> ADTIVAVELDSYPNTDIGDPNYPHIGIDIKSIRSKSTARWNMQTGKVGTVHISYNSVAKRLSAVVSYSGSSSTTVSYDVDL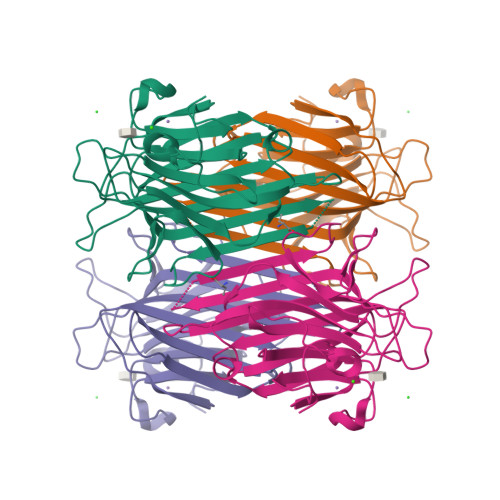NNVLPEWVRVGLSATTGLYKETNTILSWSFTSKLKTNSIADENSLHFSFHKFSQNPKDLILQGDAFTDSDGNLELTKVSNSGDPQGNSVGRALFYAPVHIWEKSAVVASFDATFTFLIKSPDREPADGITFFIANTDTSIPSGSGGRLLGLFPDAN>[2x]MTAVVKNLAKLPAATSQILTNVSKLQTFHGLLEERRDKYAPLAYHTYDNLKQKTTWHPIAHAWVDEGLPVSKKEYNEYCWLKKDMQRLLPLASPFVFGIYGILPLAVWLSNDGYLPSAFSSKKDIVSKKLEWYSSYGDDLRQQVGPMLQHRLKRHLRGTLNNEHRLMLDEVTESYKEIFYSHYTGQLRDVRKCAHLRLYDGTSTVLLLTNKEPVELTSELLQKWNAIKAAKLSPEEEKKARNEALIEAYKEQELHGGPHVKHMQGYGIPADTPLLGENAKGDQYTQPPESASIPLEQLEWTGDTVFIPAEYRTEMEDWGRELTKLANQFLLLPWRFVSNAWNQRRLVSWFEEILQEDALIAKEGGVQALSDDELKVALLDRAVIRCDEELTRGDMEARYKEISWLMSLRNPFIVLAWQTGYYRSTYSPEDDLPEASILPKLNRTVLDVDVHNELAPDHPEKPLPRVHPALYPNSHLALAKEVAVLAK;>[2x]MAAKTIPFVASTALGERLFAGVQKVLAAAKAPVSLVQTDAKFAPADAKYLLAEPLSAAATGELANKYGLSSKVTSGAASQFYPNSIYPSLNVEVVQNLYALSNPAFSSLSATTTKAVTVKDESAIKLAELQKETERNISSFFRDEANKSVQATLRLACDKAIKTKADKKTVMVVTKPHGDAFDDLLAQVTKSESDGRADELRNSSVSVEPTLVGNAWPKLVMFPEGVNVVVCGPNASGDQVAQLFVGIAGGTGMVAQQLVGDAVVFTSANAEDNENPTGALLAASNLLTALGHEAEAKKIAAAVAKAYTTDRILPKELPGGKADLEAFIDAVAKHASA;>MTHAELHLFDLDEFMQTYKRLQTRQDWLIENKCKKSRLFSYVAAVIAFTVGKSATMSDEAILAKIDPYVTSEVRVQRGAWWRSGYFTKEEVEMMTPKGPIARYYKFLLGVRRFPLKHGALSWACGFVPAWLTFTSLNHWAQNRRLNRYLTQESVFGEMARELVRGKTADEATTSVMARVEKEILGVH[2x];>[2x]MSSYTGAALAPKSERLRLAFEEKQKDHQKCIEEAKGKGLKKDELIDACAWTHRKTILALKDWFAYRPPFQDRRSKWAEYCSIRHDSGSWLGWSQKFF;>[2x]MLNSNIYIIIYGGIIMYSIMIIIQMFLYNFSNKIYIEVEINKYILSKNNIDIYWIICNCTIIIIITTLNHIINKIGIYNMIEYNICYWLIGTGLGLYISPFIVFGYKFFVYIMDLNNYSLNIYHNNNKMNDIQQIYNGTNYNDTMIFFIKDINNIFTIYRSINFFMNWLYQMIYYGVRMWLVFVLHSFSLGSFGELITVITDNNLIFNVFYIGLLGLGFILYLIVIFYLGIQIYVYISFSLSFLHSTILLFLVNYIPHYNNKSIFNTFTNKSIY;>[2x]MPSTSPADKDVPMSILHTHGLSYVNWCMSLAPGLLVFEGFFRARYYRSRVPPSRTVLMNGLKMRMFSLARQQAPKIVHKPVLSPIPEHLRLVKNVAQVQIDMLKLLNAQAAK;>MMRRACRIIRPSHVRGVSGVAPTIYLRSKAALPATSTTDVRPQLYALQRFAKAQLKTATEAERAAIEADIARYQEYLDSDLEKLKQDVAEDTAKKQKLIPLLDRYPDVPIEKIPEHANVLLKKIDACLEILSKDIGEVTDAEAHEMYFETSKFQILHIYTGCVASFPEGDVPPGAVECLPGQVIRTKVNGEDVMLEIDEVDPGYQVCWFKPDVPLPENAEILWSYPYEPTAALPTGTTWEEGQANVLIPAEPTPEAAVWPPTPVTNVYAPMAEKLALKSNPELKVLFKEALLQPAKLLPLDVDYQCSHDREVVEAKRDRYLTALVEAEQAPPLPFTPDVLQLQLEHNVLKGELIDRLRALEYTIVTEQLQARLHERRLRGDVIDEWEELDYHPLVRDDTYLAIDFGDPTFGRYIWKLFPHTDGDEECMFKDTRLDVLPPQVNPLNAILAQHTAQTPVHRSLEKRLWTEVRATAVSE[2x];>[2x]MAPLYPVLSQASLYKRHFFKNIKLFHVVFYVGAPCVTFGTAAWSGSNRNSREAIFMVIEERHGWDNFKKLSSHQQGVIMQEAAQESLLARNKGELHLP;>[2x]MVYTNWQSSYTRLFVSKPWMWHPLAWMTLSVGIWWKFGKESLCNERSFYIHTHPKWAPHKFHTVYNWSRDPIKWTLAEQYASIIRNTNTDIEAVLKIKLPANAN;>[2x]MAFGRTRPTLSSPLVPVWNDLRALQVFTSQEYMQKRGPGFTNTLEYKLSCLNPVKWYDMMKVMPGGKAFVGTALGLALFGGWGVEFVKNISVMTKEKPPIDWNNEKLGHLTRS;>LIPVSLVDLININIIFYILLLYTLLLFFIPLFLASINYTYHYIYKYYNYNYNFINNN[2x];>MSLAKVWMYASWIPRGIPKAMANELSSAAAALAHPEAIARVAQLESQGKNPYRVARAEFWQMYLACWPYRFRNTVVEWETCKAKVLKGSVDLQDIVDLLYLLAWAYLFWILGEIYGRGSLYGYRFDGEIHRQEAQNVILYKEKEAQEMAVVMEKLEKEIQEWLKTMEQE[2x];>[2x]MPLPNAVVQGYTSVRGPKRPLDHFYGRTPLNIDTLWHWVKFPHRYDNLRFAVCFWAFLVSAHFANKKQRNLRVEWEKNMEIQKKLHPSGLWSEEQAFAAAEKLGRPKAGHPMRVFEDGYQQFDLKPKLFDPDEEAHH;>[2x]MADHNKKDVGSWASPNEHLMFFDFSSWLLVDFGKRWERWVSFKKSFLTTTRSPYWSPQFFLLTFFQLRNSNVKLCENWNWAPKGDDFNLLHNSAAEPFGRDLKAHLEREAGAKHHH;>[2x]MGGDAHAAPAEKPDPALDATKALPKALEEVEFFQSYAVRRKTGFHLFNRATGSPTIVGPMFYNLYNFVRIGRVSKYVCWLSLPLVFQRMWMKNRATGMEYDIDLENYAPFEAKKNPMHGH;>MSLPTFFLAPPLTEPFRARHRRKCIEKKDTFFQCLDKNKNETEPCEVEASGYSQECPDSWRRYFNEQRWKALELKGEVKHANLKNTQQHF[2x];>MFGVTRKLLGELSEYVEVNEKGMPKPQALSLWNMPYAKRRALTKFARGVRWQFIVLFIALYNFKNRDDSHLLRRGAYN[2x];>[2x]MMRISRKLLVPVANFRPKKPWDGPWGIQISQKKDRPFIAMWILFPLLLVDHLTREYYAYWHSSKVPVTDVFGDF;>[2x]MGGKASEAVTIAFRFPHRTTFLVKQNVGQKLNKGHQTFWQLVAGGWLFFLLINRTSFKPKLAAPKV

The mitochondrial ATP synthase is a membrane protein complex that generates most of the ATP in eukaryotic cells. The translocation of protons through the membrane-bound Fo part, mediated by subunit a, drives the rotation of a membrane-embedded c-ring and the attached central stalk, which together form the rotor. The torque of the rotor against the stator subunits induces conformational changes in the (αβ)3 headpiece, thereby triggering catalysis. To reveal how the mitochondrial ATP synthase is modulated by lipids and organised into a dimer shaping discoid cristae in Euglenozoan mitochondria, we determined the structure of the ATP synthase dimer from E. gracilis.

The membrane region was determined to 2.8 Å resolution, enabling the identification of a structurally divergent subunit a and visualisation of 37 associated native lipids. The membrane-bound Fo region is composed of 22 proteins, of which 13 have no homologs in animals and fungi. The well-resolved membrane region allowed the identification of 37 native lipids, leading to the assignment of 25 cardiolipins, whereas the 12 remaining phophoslipids could not be unambiguously identified and were modelled as phosphatidic acid. Importantly, cardiolipin binding sites are found at the rotor-stator interface, dimer interface, and in a peripheral Fo cavity. Our cryo-EM map allowed tracing of subunit a, for which we identified six structurally conserved membrane-embedded helices (H1a to H6a) directly from side-chain densities. By contrast, in the E. gracilis structure, the N-terminal part of H5a is kinked towards the lumen, and therefore does not interact with the c-ring, and instead extends towards the lumenal membrane surface. This structural rearrangement results in a smaller interface between subunits a and c, with only three c-subunits forming interactions, which also has implications for the formation of the matrix half-channel. At the exit of the lumenal half-channel, we identified a β-DDM detergent molecule, with its hydrophilic maltose head group protruding into the channel and the acyl chain extending between H5a and H6a, confirming both the hydrophilic environment and accessibility of the membrane-intrinsic lumen channel. Adjacent to the proton-half channels, the E. gracilis ATP synthase structure reveals two bound cardiolipins (CDL1, CDL2) flanking either side of the two horizontal helices H5a and H6a. Near the matrix half-channel, CDL2 is coordinated collectively by R160 of H5a, R50 of ATPEG6 and R22 of subunit k. Together, these two bound cardiolipins enclose the two horizontal membrane helices H5a and H6a, possibly acting to seal the Fo against proton leakage by recruiting a high density of acyl chains, as well as separating lipid and aqueous environments in the vicinity of the two half-channels.>[4x]MKRMLINATQQEELRVALVDGQRLYDLDIESPGHEQKKANIYKGKITRIEPSLEAAFVDYGAERHGFLPLKEIAREYFPANYSAHGRPNIKDVLREGQEVIVQIDKEERGNKGAALTTFISLAGSYLVLMPNNPRAGGISRRIEGDDRTELKEALASLELPEGMGLIVRT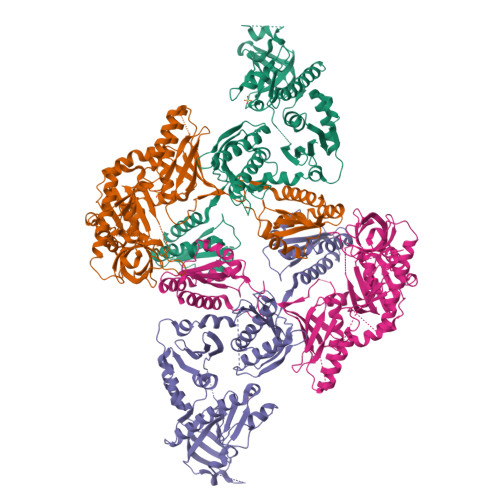AGVGKSAEALQWDLSFRLKHWEAIKKAAESRPAPFLIHQESNVIVRAFRDYLRQDIGEILIDNPKVLELARQHIAALGRPDFSSKIKLYTGEIPLFSHYQIESQIESAFQREVRLPSGGSIVIDSTEALTAIDINSARATRGGDIEETAFNTNLEAADEIARQLRLRDLGGLIVIDFIDMTPVRHQRAVENRLREAVRQDRARIQISHISRFGLLEMSRQRLSPSLGESSHHVCPRCSGTGTVRDNESLSLSILRLIEEEALKENTQEVHAIVPVPIASYLLNEKRSAVNAIETRQDGVRCVIVPNDQMETPHYHVLRVRKGEETPTLSYMLPKLHEEAMALPSE>GPGSMAHSAHDDADNDTEYRIEHDTMGEVRVPAKALWRAQTQRAVENFPISGRGLERAQIRALGLLKGACAQVNMDLGLLAPEKAEAIIAAAAEIADGQHDDQFPIDVFQTGSGTSSNMNTNEVIASIAGANGVAVHPNDDVNMSQSSNDTFPTATHIAATEAAVSHLIPALEILQDALATKALEWQSVVKSGRTHLMDAVPVTLGQEFSGYARQIEAGIERVRATLPRLGELAIGGTAVGTGLNAPEGFGVKVVSVLVSQTGLPQLRTAANSFEAQAARDGLVEASGALRTIAVSLTKIANDIRWMGSGPLTGLAEIQLPDLQPGSSIMPGKVNPVLPEAVTQVAAQVIGNDAAVAWGGANGAFELNVYIPMMARNILESFTLLTNVSKLFAQRCIAGLTANAEHLRELAESSPSIVTPLNSAIGYEEAAAVAK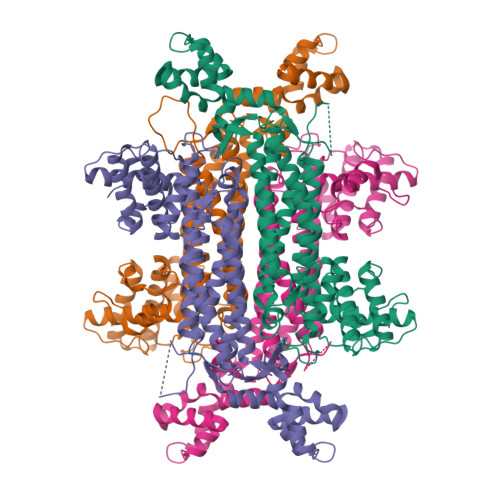QALKERKTIRQTVIDRGLIGDKLSLEELDRRLDVLAMAKVEAT[4x]1-ACETYL-4-(4-{4-[(2-ETHOXYPHENYL)THIO]-3-NITROPHENYL}PYRIDIN-2-YL)PIPERAZINE | C25 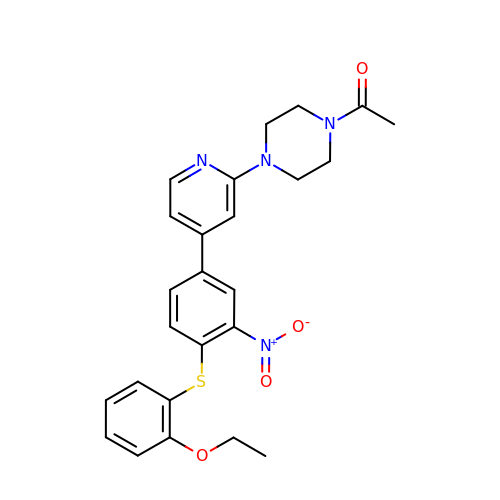H26 N4 O4 S | GKGJFUXSTSUKPB-UHFFFAOYSA-N>NGNSLSAAELTCGMIMCLARQIPQATASMKDGKWERKKFMGTELNGKTLGILGLGRIGREVATRMQSFGMKTIGYDPIISPEVSASFGVQQLPLEEIWPLCDFITVHTPLLPSTTGLLNDNTFAQCKKGVRVVNCARGGIVDEGALLRALQSGQCAGAALDVFTEEPPRDRALVDHENVISCPHLGASTKEAQSR[2x]

Human 3-phosphoglycerate dehydrogenase (PHGDH) is responsible for the NAD+-dependent conversion of 3-phosphoglycerate (3-PG) to phosphohydroxypyruvate (PHP), which is the first step in the de novo serine synthesis pathway. Thus, PHGDH activity diverts glycolytic flux into biomass production. Limited proteolysis with thermolysin revealed a stable fragment of PHGDH consisting of the core of the catalytic domain containing the cofactor-binding site, and this was shown to crystallise readily. Thus PHGDH-93 provides a valuable tool to investigate binders to the cofactor-binding site.

PHGDH-93 was then successfully crystallised with an empty, accessible cofactor-binding pocket. Soaking of all 15 fragments into PHGDH-93 crystals was performed overnight at RT using a fragment concentration of 80 mM in 20 % DMSO. Difference electron density corresponding to seven fragments (3, 5, 9, 10, 14-16, 47 % of tested compounds) was clearly visible. All of the fragments for which crystallographic data were obtained bound to the adenine-pocket suggesting this pocket to be a preferential site for fragment binding. Analysis of the fragments’ binding modes showed that four of the fragments (5, 14, 15 and 16) were coordinated by hydrogen and/or halogen bonds, whereas the other three fragments (3, 9 and 10) appeared to be stabilised only by apolar contacts. The remaining two crystallographically observed fragments, 3 (1-methyl-3-phenyl-1H-pyrazol-5-amine) and 10 (3-(1,3-oxazol-5-yl)aniline) were non-fused bicyclic aromatic systems, which, although not forming specific hydrogen bonds to the protein, bound in a similar orientation to one another to the adenine pocket (3, Kd = 5.8 ± 2.0 mM and 10, Kd = 9.3 ± 3.8 mM).> A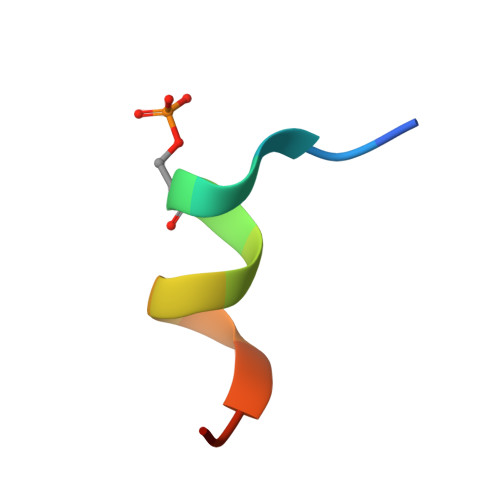RRESYLKATQPSL> MSFLFSSRSSKTFKPKKNIPEGSHQYELLKHAEATLGSGNLRQAVMLPEGEDLNEWIAVNTVDFFNQINMLYGTITEFCTEASCPVMSAGPRYEYHWADGTNIKKPIKCSAPKYIDYLMTWVQDQLDDETLFPSKI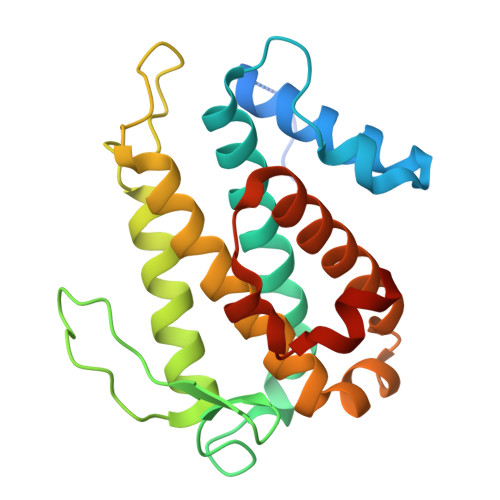GVPFPKNFMSVAKTILKRLFRVYAHIYHQHFDSVMQLQEEAHLNTSFKHFIFFVQEFNLIDRRELAPLQELIEKLGSKDR In this work, we exhaustively probe the ability of all 36 immobile HJ sequences to form DNA crystals in two different designed systems. Three separate self-assembling DNA crystal systems are described in this report: the “4 × 5” and “4 × 6” designs (collectively referred to as the 4 × N systems), and a third construct with a “scrambled” sequence variant of the 4 × 6 lattices. Self-assembly was mediated by three constituent oligonucleotides: (S1) containing four sequence repeats of either 5 or 6 bases; (S2) composed of 21 bases containing complementary regions to both (S1); and (S3) which forms the second junction crossover. The HJ serves as the fundamental component at the core of each unit, and the ultimate assembly of the full lattice is facilitated by the complementary 2-base sticky ends that tail each duplex.

Because the 4 × 6 system yielded R3 symmetry in 5 of 17 junctions, we considered whether the downstream sequences adjacent to the junction could play a role in crystallization efficiency, junction angle, and symmetry preference, or if the HJ alone was the singular determinant. To investigate this possibility, we designed “scrambled” sequences with targeted base substitutions, while maintaining GC content, along each “stem”. Contrary to the buffer preference observed with the native P32 crystals, the scrambled systems exhibited an exclusive preference towards low salt buffers, much like the native R3 crystals. Remarkably, only J1 and J2 retained the P32 symmetry, with all others yielding an R3 lattice. There appeared to be only a marginal difference in the average cell lengths in the R3 scramble crystals (a = b = 113.04 c = 51.10) relative to the native 4 × 6 sequences: the a, b axis trended ~2 Å shorter and c ~1.3 Å longer, whereas in the J1 and J2 cases, the crystals were in good agreement with the original 4 × 6 motif. The average angles of the R3 and P32 crystals were 61.00° (σ = 1.21) and 58.05° (σ = 1.39), respectively. Further, we observed modest improvements in resolution, reaching as high as 2.7 Å in J36. Notably, all junctions preventing crystallization compared to its original counterpart remained fatal and all relative cavity dimensions and volumes remained unperturbed. However, in the majority of the crystal structures reported here, the cacodylate anion indeed fits best into the electron density map of our X-ray structures, due to the presence of sodium cacodylate in the crystallization solution.

> CCGTCG;> GAACGACACCGACGGGGACTC;> TCGAGTCC;> GTGTCGT> MQNGDFQILDYTGLISTMPRVDTLLQSMNLFTEHFGRTTVARIERLDDGAGDIKAVQRGGVRQHLANDRKKIVNLNIPFFPLDRSIDRADIQNFREFGTENAPATVDAEVQRHMARIRRSHAILKSKAMYAALKGTSWSPDDPVSDYNYYDVWGATQTTADVDFTKLGVDPIEVLEAEARAHIIDWAGDNGDNYEIVVLASRQWFSALIAHPQVTGAYSQYPSTQEILRRRLGGNANNRIFEHKNILFIEDISGNIPAGEAYIFPRGISRMFEIYYAPSDTLRDANQAAQE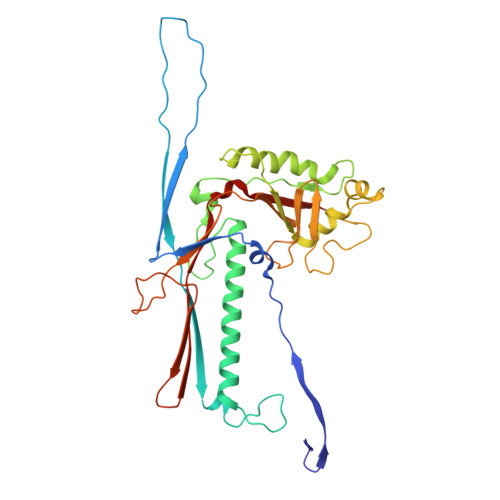LYVFFKESNYLREAKIESETSFLTVNNRPELVVKSTGKFTA cyclopropanecarboxylic acid | C4 H6 O2 | 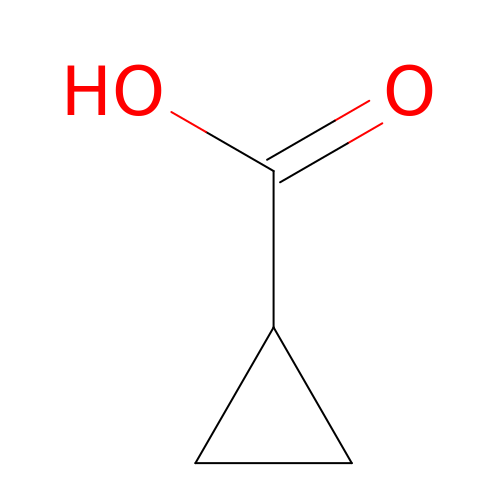YMGUBTXCNDTFJI-UHFFFAOYSA-N> GPDSMSTFIFPGDSFPVDPTTPVKLGPGIYCDPNTQEIRPVNTGVLHVSAKGKSGVQTAYIDYSSKRYIPSVNDFVIGVIIGTFSDSYKVSLQNFSSSVSLSYMAFPNASKKNRPTLQVGDLVYARVCTAEKELEAE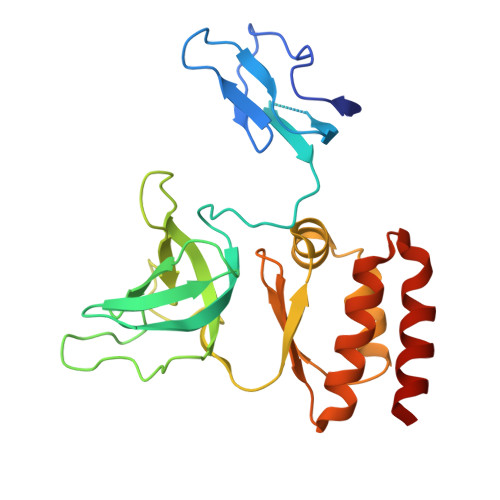IECFDSTTGRDAGFGILEDGMIIDVNLNFARQLLFNNDFPLLKVLAAHTKFEVAIGLNGKIWVKCEELSNTLACYRTIMECCQKNDTAAFKDIAKRQFKEILTVKEE>MADPRPDPDELARRAAQVIADRTGIGEHDVAVVLGSGWLPAVAALGSPTTVLPQAELPGFVPPTAAGHAGELLSVPIGAHRVLVLAGRIHAYEGHDLRYVVHPVRAARAAGAQIMVLTNAAGGLRADLQVGQPVLISDHLNLTARSPLVGGEFVDLTDAYSPRLRELARQSDPQLAEGVYAGLPGPHYETPAEIRMLQTLGADLVGMSTVHETIAARAAGAEVLGVSLVTNLAAGITGEPLSHAEVLAAGAASATRMGALLADV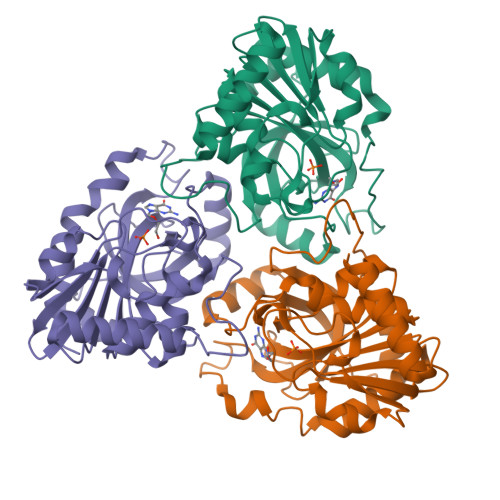IARF[3x]>[2x]MDVVSLDKPFMYFEEI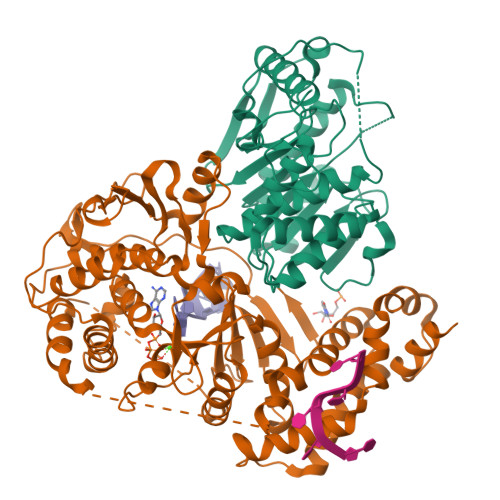DNELDYEPESANEVAKKLPYQGQLKLLLGELFFLSKLQRHGILDGATVVYIGSAPGTHIRYLRDHFYNLGVIIKWMLIDGRHHDPILNGLRDVTLVTRFVDEEYLRSIKKQLHPSKIILISDVASAAGGNEPSTADLLSNYALQNVMISILNPVASSLKWRCPFPDQWIKDFYIPHGNKMLQPFAPSYSAEMRLLSIYTGENMRLTRVTKSDAVNYEKKMYYLNKIVRNKVVVNFDYPNQEYDYFHMYFMLRTVYCNKTFPTTKAKVLFLQQSIFRFLNIP;>MNRNPDQNTLPNITLKIIETYLGRVPSVNEYHMLKSQARNIQKITVFNKDIFVSLVKKNKKRFFSDVNTSASEIKDRILSYFSKQTQTYNIGKLFTIIELQSVLVTTYTDILGVLTIKAPNVISSKISYNVTSMEELARDMLNSMNVAVIDKAKVMGRHNVSSLVKNVNKLMEEYLRRHNKSCICYGSYSLYLINPNIRYGDIDILQTNSRTFLIDLAFLIKFITGNNIILSKIPYLRNYMVIKDENDNHIIDSFNIRQDTMNVVPKIFIDNIYIVDPTFQLLNMIKMFSQIDRLEDLSKDPEKFNARMATMLEYVRYTHGIVFDGKRNNMPMKCIIDENNRIVTVTTKDYFSFKKCLVYLDENVLSSDILDLNADTSCDFESVTNSVYLIHDNIMYTYFSNTILLSDKGKVHEISARGLCAHILLYQMLTSGEYKQCLSDLLNSMMNRDKIPIYSHTERDKKPGRHGFINIEKDIIVF[2x]>[4x]FACKTANGTAIPIGGGSANVYVNLAPVVNVGQNLVVDLSTQIFCHNDYPETITDYVTLQRGSAYGGVLSNFSGTVKYSGSSYPFPTTSETPRVVYNSRTDKPWPVALYLTP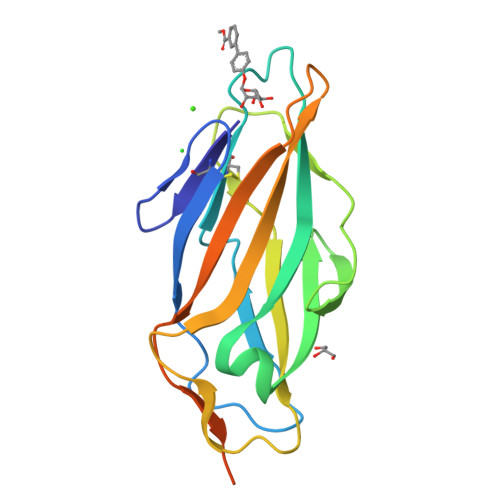VSSAGGVAIKAGSLIAVLILRQTNNYNSDDFQFVWNIYANNDVVVPTGGCDVSARDVTVTLPDYHHHHHH>ESARSQVQVHAPVVAARLRNIWPKFPKWLHEAPLAVAWEVTRLFMHCKVDLEDESLGLKYDPSWSTARDVTDIWKTLYRLDAFRGKPFPEKPPNDVFVTAMTGNFESKGSAVVLSAVLDYNPDNSPTAPLYLVKLKPLMFEQGCRLTRRFGPDRFFEILIPSPTSTSPSVPPVVSKQPAAVEEVIQWLTMGQHSLVGRQWRAFFAKDAGYRKPLREFQLRAEDPKPIIKERVHFFAETGITFRPDVFKTRSVVPAEEPVEQRTEFKVSQMLDWLLQLDNNTWQPHLKLFSRIQLGLSKTYAIMTLEPHQIRHHKTDLLSPSGTGEVMNDGVGRMSRSVAKRIRDVLGLGDVPSAVQGRFGSAKGMWVIDVDDTGDEDWIETYPSQRKWECDFVDKHQRTLEVRSVASELKSAGLNLQLLPVLEDRARDKVKMRQAIGDRLINDLQRQFSEQKHALNRPVEFRQWVYESYSSRATRVSHGRVPFLAGLPD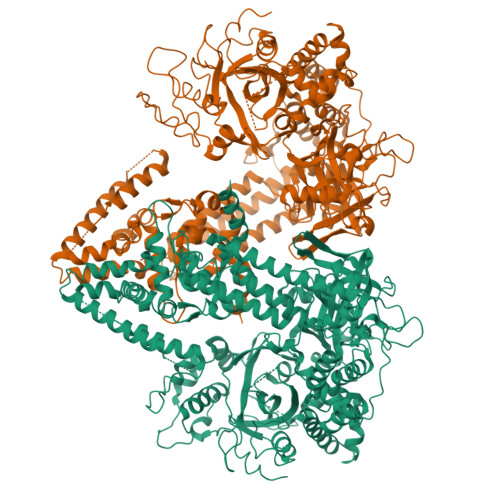SQEETLNFLMNSGFDPKKQKYLQDIAWDLQKRKCDTLKSKLNIRVGRSAYIYMIADFWGVLEENEVHVGFSSKFRDEEESFTLLSDCDVLVARSPAHFPSDIQRVRAVFKPELHSLKDVIIFSTKGDVPLAKKLSGGDYDGDMAWVCWDPEIVDGFVNAEMPLEPDLSRYLKKDKTTFKQLMASHGTGSAAKEQTTYDMIQKSFHFALQPNFLGMCTNYKERLCYINNSVSNKPAIILSSLVGNLVDQSKQGIVFNEASWAQLRRELLGGALSLPDPMYKSDSWLGRGEPTHIIDYLKFSIARPAIDKELEAFHNAMKAAKDTEDGAHFWDPDLASYYTFFKEISDKSRSSALLFTTLKNRIGEVEKEYGRLVKNKEMRDSKDPYPVRVNQVYEKWCAITPEAMDKSGANYDSKVIRLLELSFLADREMNTWALLRASTAFKLYYHKSPKFVWQMAGRQLAYIKAQMTSRPGEGAPALMTAFMYAGLMPDKKFTKQYVARLEGDGSEYPDPEVYEVLGDDDFDGIGFTGNGDY[2x]> DRVYIHPFHLLYHNKSTCAQLENPSVETLPESTFEPVPIQAKTSPVNEKTLHDQLVLAAEKLEDEDRKRAAQVAMITNFVGFRMYKMLNEAGSGASGAILSPPALFGTLVSFYLGSLDPTASQLQTLLDVPVKEGDCTSRLDGHKVLAALRAVQGLLVTQGGSS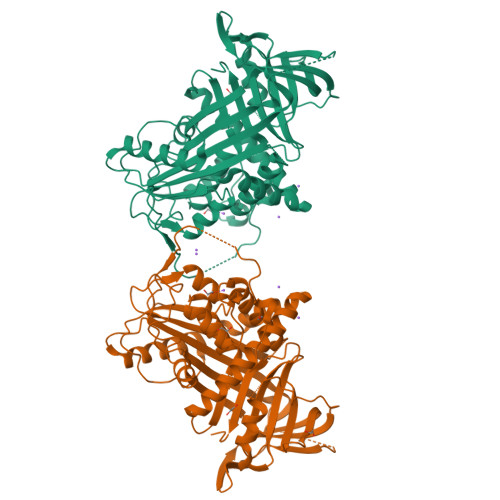SQTPLLQSIVVGLFTAPGFRLKHSFVQSLALFTPALFPRSLDLSTDPVLATEKINRFIKAVTGWKMNLPLEGVSTDSTLLFNTYVHFQGTMRGFSQLPGVHEFWVDNSISVSVPMISGTGNFQHWSDAQNNFSVTCVPLGERATLLLIQPHCISDLDRVEALIFQNDLLTWIENPPPRAIRLTLPQLEIRGSYNLQDLLAEDKLPTLLGAEANLNNIGDTNPRVGEVLNSILLELKAGEEEQPTTSVQQPGSPEALDVTLSSPFLFAIYEQDSGTLHFLGRVNNPQSVV>MVEAPEQSETGRIEAFSDGVFAIAITLLVLEIKVPQHKIVETVGLVSSLLSLWPSYLAFLTSFASILVMWVNHHRIFSLVARTDHAFFYWNGLLLMLVTFVPFPTALLAEYLIHPQARVAASVYAGIFLAIAIVFNRLWKHAATADRLLAQKADRHEVDAITKQYRFGPGLYLVAFALSFISVWLSVGVCFVLAIYFALRSN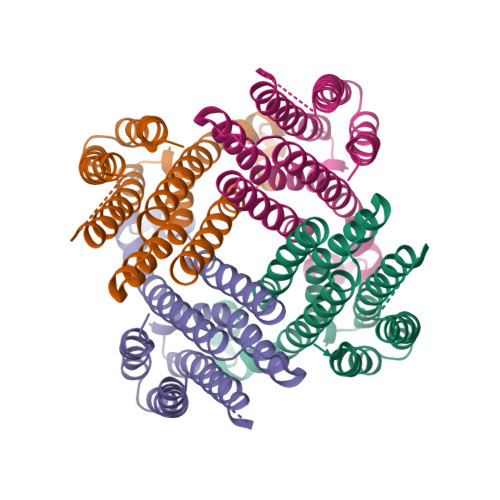A[4x]> MASNYNS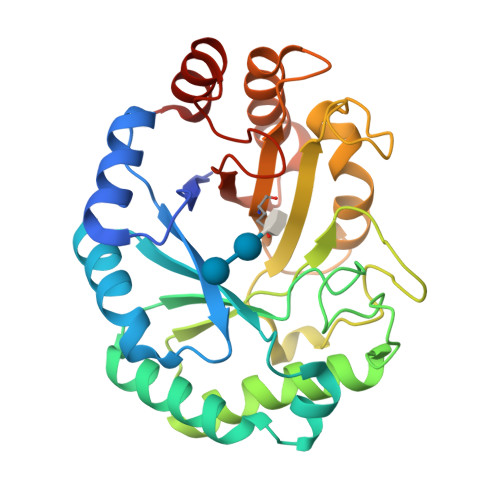GLKIGAWVGTQPSESAIKSFQELQGRKLDIVHQFINWSTDFSWVRPYADAVYNNGSILMITWEPWEYNTVDIKNGKADAYITRMAQDMKAYGKEIWLRPLHAANGDWYPWAIGYSSRVNTNETYIAAFRHIVDIFRANGATNVKWVFNVNCDNVGNGTSYLGHYPGDNYVDYTSIDGYNWGTTQSWGSQWQSFDQVFSRAYQALASINKPIIIAEFASAEIGGNKARWITEAYNSIRTSYNKVIAAVWFHENKETDWRINSSPEALAAYREAIGA> SKLTDPLYIKKICLEKVHDWSRCNEDDVCVNQILSGLTNQLFEVSIKEDTAIEYRITRRHVLFRIYGKDVDALYNPLSEFEVYKTMSKYRIAPLLLNTFDGGRIEEWLYGDPLSIDDLKNKSILVGIANVLGKFHTLSRKRHLPEHWDKTPCVFKMMDRWRLAVSNYKNLDKVTLDINKYIQESHKFLKFIKIYT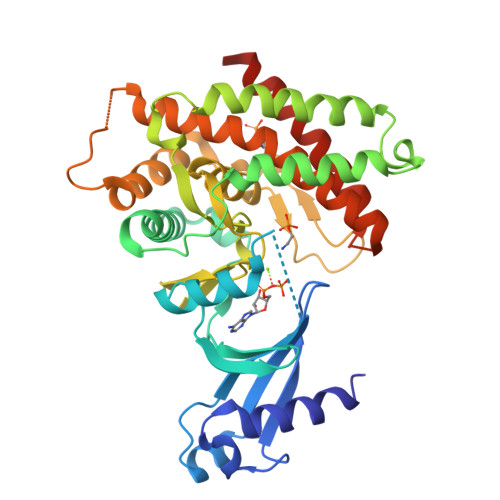QIENIANDIVFCHNDLQENNIMNTNKCLRLIDFEYSGYNFLSADIANFFIETTIDYSYNAYPFFIINKKNYISYESRILFVTTYLSKYLDDSTAASDQDIIDQFLEAIEVQALGLHLIWAFWSIIRGYQTKSYNEFDFFLYAKERLKMYDEQKQYLMSKNIIKDYDD3-TRIMETHYLSILYLSUCCINIC ACID 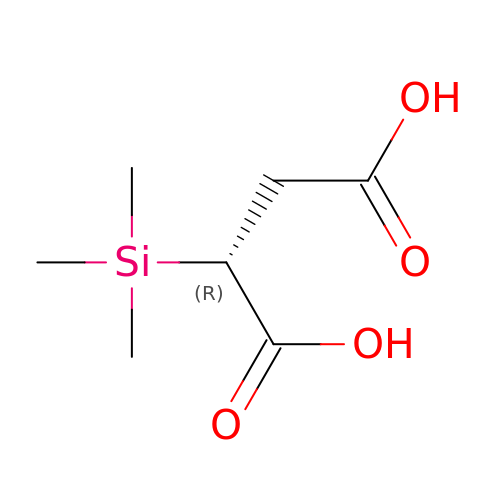| C7 H14 O4 Si | RTXZCZFAAYFFKF-UHFFFAOYSA-N>GTSSMADIGSTNDALDYYLKSKGFNGLFSQIELSFSASNLRDRDVLSKSDPMVVVYQKEKDATLSEVFRSEVVLNSLAPKWIKKFIVAYHFETVQTLVFRVYDVDTKFQNSREEMLKLDEQQFLGEATCALSEIITKSTRTSTLELKRKDGFAPQAQPHHGKLIIHAEESLASKISTEIVFRCSNLESKDLFSKSDPFLVVSKIVEHGTPIPVSKTEVRKNDLNPIWKPVFLSVQQVGSKDSPVIIECSDFNSNGKHSLIGKVQKSLSDLEKLHLAGQGINFSLPTGAGQNKVLKSQLFVDKFTETVHHTFLEYLASGFELNFMVAIDFTASNGNPRLPDSLHYIDPSGRLNAYQRAIMDVGEVLQFYDSDKRFPAWGFGARPIDAPVSHCFNLNGSSSYSEVDGIQGIMTSYTSALFNVSLAGPTLFGPVINAAAMIASASLAQGSRKYYVLLIITDGVITDLQETKDALVSASDLPLSILIVGVGGADFKEMEILDADKGERLESSSGRLASRDIVQFVALRDVQYGEISVVQALLAELPSQFLTYMRIRN[4x];> GLFSQIELSFSASNLRDRDVLSKSDPMVVVYQKEKDATLSEVFRSEVVLNSLAPKWIKKFIVAYHFETVQTLVFRVYDVDTKFQNSREEMLKLDEQQFLGEATCALSEIITKSTRTSTLELKRKDGFAPQAQPHHGKLIIHAEESLASKISTEIVFRCSNLESKDLFSKSDPFLVVSKIVEHGTPIPVSKTEVRKNDLNPIWKPVFLSVQQVGSKDSPVIIECSDFNSNGKHSLIGKVQKSLSDLEKLHLAGQGINFSLPTGAGQNKVLKSQLFVDKFTETVHHTFLEYLASGFELNFMVAIDFTASNGNPRLPDSLHYIDPSGRLNAYQRAIMDVGEVLQFYDSDKRFPAWGFGARPIDAPVSHCFNLNGSSSYSEVDGIQGIMTSYTSALFNVSLAGPTLFGPVINAAAMIASASLAQGSRKYYVLLIITDGVITDLQETKDALVSASDLPLSILIVGVGGADFKEMEILDADKGERLESSSGRLASRDIVQFVALRDVQYGEISVVQALLAELPSQFLTYMRIRN;> SMADIGSTNDALDYYLKSKGFNGLFSQIELSFSASNLRDRDVLSKSDPMVVVYQKEKDATLSEVFRSEVVLNSLAPKWIKKFIVAYHFETVQTLVFRVYDVDTKFQNSREEMLKLDEQQFLGEATCALSEIITKSTRTSTLELKRKDGFAPQAQPHHGKLIIHAEESLASKISTEIVFRCSNLESKDLFSKSDPFLVVSKIVEHGTPIPVSKTEVRKNDLNPIWKPVFLSVQQVGSKDSPVIIECSDFNSNGKHSLIGKVQKSLSDLEKLHLAGQGINFSLPTGAGQNKVLKSQLFVDKFTETVHHTFLEYLASGFELNFMVAIDFTASNGNPRLPDSLHYIDPSGRLNAYQRAIMDVGEVLQFYDSDKRFPAWGFGARPIDAPVSHCFNLNGSSSYSEVDGIQGIMTSYTSALFNVSLAGPTLFGPVINAAAMIASASLAQGSRKYYVLLIITDGVITDLQETKDALVSASDLPLSILIVGVGGADFKEMEILDADKGERLESSSGRLASRDIVQFVALRDVQYGEISVVQALLAELPSQFLTYMRIRN;> LFSQIELSFSASNLRDRDVLSKSDPMVVVYQKEKDATLSEVFRSEVVLNSLAPKWIKKFIVAYHFETVQTLVFRVYDVDTKFQNSREEMLKLDEQQFLGEATCALSEIITKSTRTSTLELKRKDGFAPQAQPHHGKLIIHAEESLASKISTEIVFRCSNLESKDLFSKSDPFLVVSKIVEHGTPIPVSKTEVRKNDLNPIWKPVFLSVQQVGSKDSPVIIECSDFNSNGKHSLIGKVQKSLSDLEKLHLAGQGINFSLPTGAGQNKVLKSQLFVDKFTETVHHTFLEYLASGFELNFMVAIDFTASNGNPRLPDSLHYIDPSGRLNAYQRAIMDVGEVLQFYDSDKRFPAWGFGARPIDAPVSHCFNLNGSSSYSEVDGIQGIMTSYTSALFNVSLAGPTLFGPVINAAAMIASASLAQGSRKYYVLLIITDGVITDLQETKDALVSASDLPLSILIVGVGGADFKEMEILDADKGERLESSSGRLASRDIVQFVALRDVQYGEISVVQALLAELPSQFLTYMRIRN;> GTSSMADIGTTNDALDYYLKSKGFNGLFSQIELSFSASNLRDRDVLSKSDPMVVVYQKEKDATLSEVFRSEVVLNSLAPKWIKKFIVAYHFETVQTLVFRVYDVDTKFQNSREEMLKLDEQQFLGEATCALSEIITKSTRTSTLELKRKDGFAPQAQPHHGKLI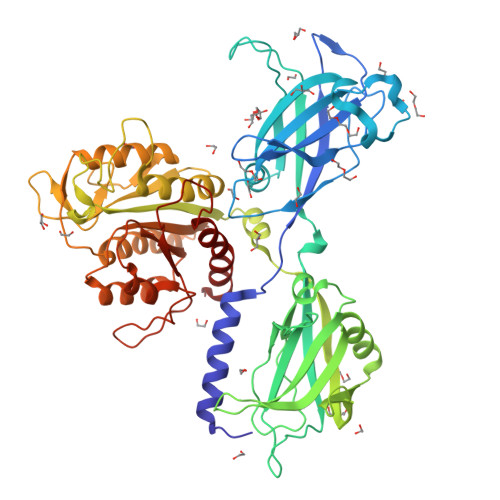IHAEESLASKISTEIVFRCSNLESKDLFSKSDPFLVVSKIVEHGTPIPVSKTEVRKNDLNPIWKPVFLSVQQVGSKDSPVIIECSDFNSNGKHSLIGKVQKSLSDLEKLHLAGQGINFSLPTGAGQNKVLKSQLFVDKFTETVHHTFLEYLASGFELNFMVAIDFTASNGNPRLPDSLHYIDPSGRLNAYQRAIMDVGEVLQFYDSDKRFPAWGFGARPIDAPVSHCFNLNGSSSYSEVDGIQGIMTSYTSALFNVSLAGPTLFGPVINAAAMIASASLAQGSRKYYVLLIITDGVITDLQETKDALVSASDLPLSILIVGVGGADFKEMEILDADKGERLESSSGRLASRDIVQFVALRDVQYGEISVVQALLAELPSQFLTYMRIRN>MSQLAHNLTLSIFDPVANYRAARIICTIGPSTQSVEALKGLIQSGMSVARMNFSHGSHEYHQTTINNVRQAAAELGVNIAIALDTKGPEIRTGQFVGGDAVMERGATCYVTTDPAFADKGTKDKFYIDYQNLSKVVRPGNYIYIDDGILILQVQSHEDEQTLECTVTNSHTISDRRGVNLPGCDVDLPAVSAKDRVDLQFGVEQGVDMIFASFIRSAEQVGDVRKALGPKGRDIMIICKIENHQGVQNIDSIIEESDGIMVARGDLGVEIPAEKVVVAQKILISKCNVAGKPVICATQMLESMTYNPRPTRAEVSDVANAVFNGADCVMLSGETAKGKYPNEVVQYMARICLEAQSALNEYVFFNSIKKLQHIPMSADEAVCSSAVNSVYETKAKAMVVLSNTGRSARLVAKYRPNCPIVCVTTRLQTCRQLNITQGVESVFFDADKLG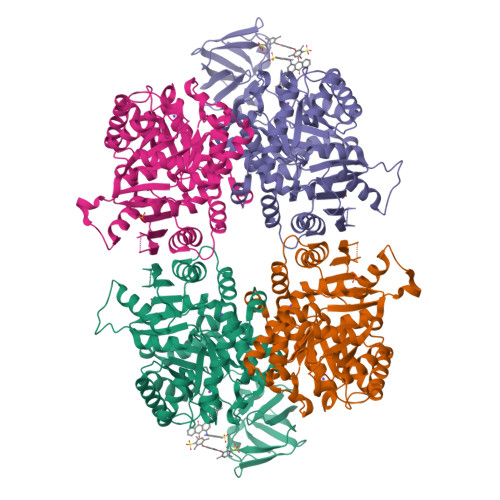HDEGKEHRVAAGVEFAKSKGYVQTGDYCVVIHADHKVKGYANQTRILLVE[2x]>GAMKSQEYTLIKIFVSNVKDFYSIFMNSIRSSQSVLNACIEKKEAPNNNNNKINNNKINNNKINNNKINNNKSNNNKSNNNNNCGSSANISNTFFTDFEKGEEDLKNKIWNEDFFVKDKKVIFLGSTLKPETAYGQNYTFINPNEYYYLTLGFDKQNLHYGDKSYVNNIMT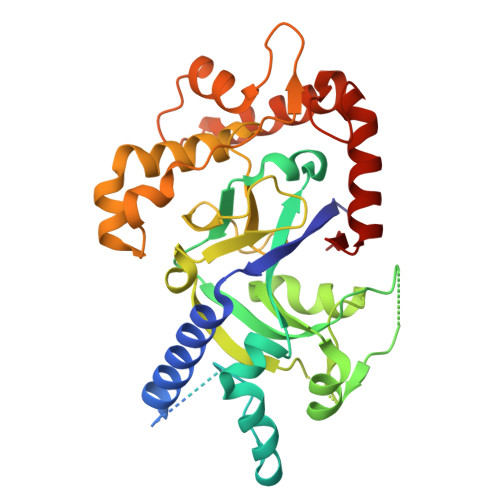KEEIINSCPNIYVCSENSLYNLAYQGIIPLLKNKNGNLDDVFILNKIKGEHFVGLETYTNISKIKNLYILPMTTIKMNISTGIVPCVSSDSTDDYACLEDIRKKKNYYCEKYNLKEEQLKNNSESCIELPEIGNNTGKYYYEKEKVSSYKDVKLQKIKEVLYKKQYFEGIMTVDPYKGMKTFNCRKLAKQNIIRNLDGFLYSE[2x]>XGELAALKELAALKELAA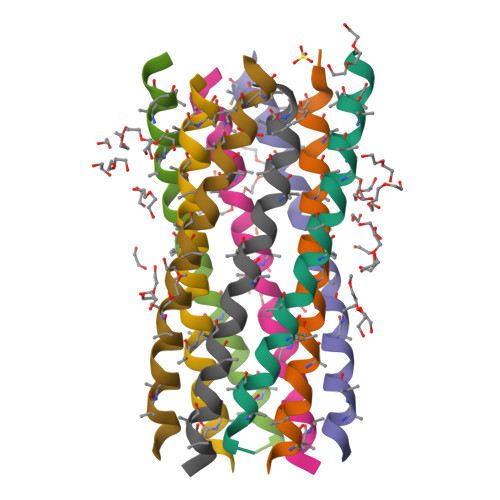LKELAALKAAAXKGX[8x]>[2x]MGENMKKKVVIIGGGAAGMSAASRVKRLKPEWDVKVFEATEWVSHAPCGIPYVVEGLSTPDKLMYYPPEVFIKKRGIDLHLNAEVIEVDTGYVRVRENGGEKSYEWDYLVFANGASPQVPAIEGVNLKGVFTADLPPDALAIREYMEKYKVENVVIIGGGYIGIEMAEAFAAQGKNVTMIVRGERVLRRSFDKEVTDILEEKLKKHVNLRLQEITMKIEGEERVEKV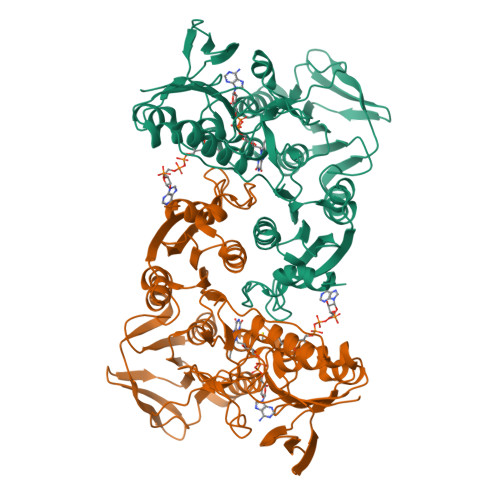VTDAGEYKAELVILATGIKPNIELAKQLGVRIGETGAIWTNEKMQTSVENVYAAGDVAETRHVITGRRVWVPLAPAGNKMGYVAGSNIAGKELHFPGVLGTAVTKFMDVEIGKTGLTEMEALKEGYDVRTAFIKASTRPHYYPGGREIWLKGVVDNETNRLLGVQVVGSDILPRIDTAAAMLMAGFTTKDAFFTDLAYAPPFAPVWDPLIVLARVLKFLEHHHHHH> MLIGYVRVATNDQNTDLQRNALVCAGCEQIFEDKLSGTRTDRPGLKRALKRLQKGDTLVVWKLDRLGRSMKHLISLVGELRERGINFRSLTDSIDTSSPMGRFFFHVMGALAEVERELIIERTMAGLAAARNKGRIGGRPPKLTKAEWEQAGRLLAQGIPRKQVALIYDVA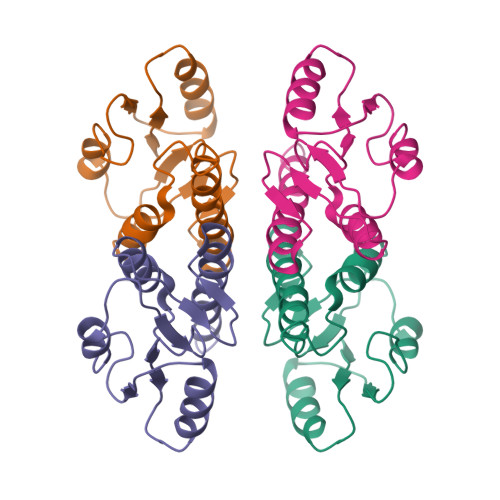LSTLYKKHPAKRAHIENDDRIN>ACRQEPQPQGPPPAAGAVASYDYLVIGGGSGGLASARRAAELGARAAVVESHKLGGTCVNVGCVPKKVMWNTAVHSEFMHDHADYGFPSCEGKFNWRVIKEKRDAYVSRLNAIYQNNLTKSHIEIIRGHAAFTSDPKPTIEVSGKKYTAPHILIATGGMPSTPHESQIPGASLGITSDGFFQLEELPGRSVIVGAGYIAVEMAGILSALGSKTSLMIRHDKVLRSFDSMISTNCTEELENAGVEVLKFSQVKEVKKTLSGLEVSMVTAVPGRLPVMTMIPDVDCLLWAIGRVPNTKDLSLNKLGIQTDDKGHIIVDEFQNTNVKGIYAVGDVCGKALLTPVAIAAGRKLAHRLFEYKEDSKLDYNNIPT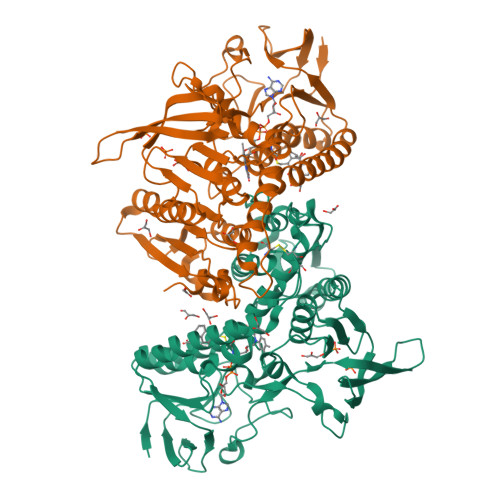VVFSHPPIGTVGLTEDEAIHKYGIENVKTYSTSFTPMYHAVTKRKTKCVMKMVCANKEEKVVGIHMQGLGCDEMLQGFAVAVKMGATKADFDNTVAIHPTSSEELVTLR[2x]>[12x]GEGLTIDLKNFRKPGEKTFTQRSRLFVGNLPPDITEEEMRKLFEKYGKAGEVFIHKDKGFGFIRLETRTLAEIAKVELDNM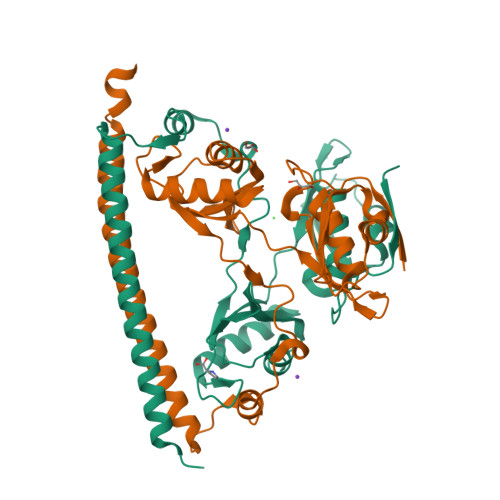PLRGKQLRVRFACHSASLTVRNLPQYVSNELLEEAFSVFGQVERAVVIVDDRGRPSGKGIVEFSGKPAARKALDRCSEGSFLLTTFPRPVTVEPMDQLDDEEGLPEKLVIKNQQFHKEREQPPRFAQPGSFEYEYAMRWKALIEMEKQQQDQVDRNIKEAREKLEMEMEAARHEHQVMLM>GPLGSPEGTLGSCSSSSECLEDSTMGSVADTVARVLRGCLENMPEADCIPKEQLSTSFQWVTKWVDYSNK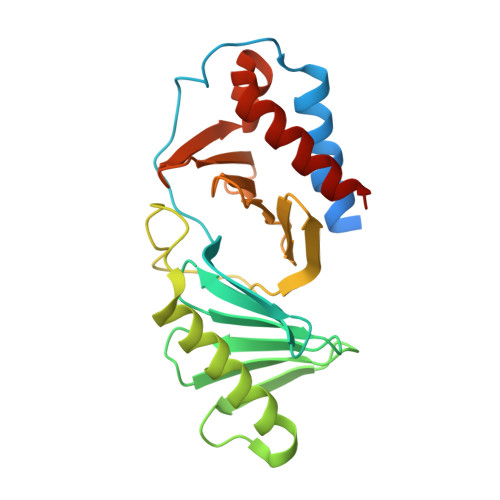YGFGYQLSDHTVGVLFNNGAHMSLLPDKKTVHYYAELGQCSVFPATDAPEQFISQVTVLKYFSHYMEENLMDGGDLPSVTDIRRPRLYLLQWLKSDKALMMLFNDGTFQVNFYHDHTKIIICSQNEEYLLTYINEDRISTTFRLTTLLMSGCSSELKNRMEYALNMLLQRCN[2x]> DISTLPRVKVDLVKPPFVHAHDQVAKTGPRVVEFTMTIEEKKLVIDREGTEIHAMTFNGSVPGPLMVVHENDYVELRLINPDTNTLLHNIDFHAATGALGGGALTQVNPGEETTLRFKATKPGVFVYHCAPEGMVPWHVTSGMNGAIMVLPRDGLKDEKGQPLTYDKIYYVGEQDFYVPKD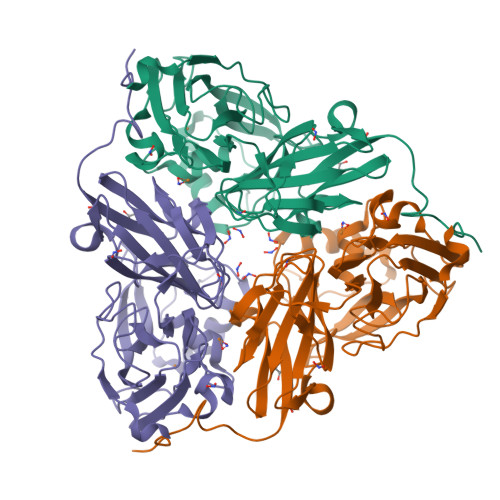EAGNYKKYETPGEAYEDAVKAMRTLTPTHIVFNGAVGALTGDHALTAAVGERVLVVHSQANRDTRPHLIGGHGDYVWATGKFRNPPDLDQETWLIPGGTAGAAFYTFRQPGVYAYVNHNLIEAFELGAAGHFKVTGEWNDDLMTSVVKPAS> MVKNNLGVAVIGSKQYAVNLLWGSSQDTETTNQALNKSLTLMSSKLYSVIGRFQGEQFAVGDKNIGHKRGQVTLLSAIDFDGSSFCGLFPADNELWLVIGVDKDGMVH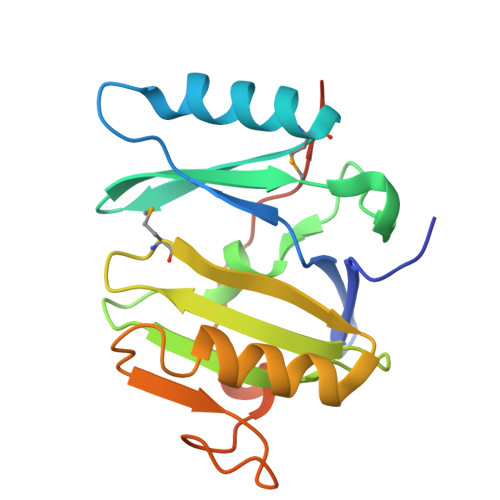FDKSFHSKDDAKKFFFDHVAYGYPWDRTYSPSDVGVGESRSISELSLIKGKKLKEKGSHHHHHH> MASMTGGQQMGRDQAGITGTWYNQLGSTFIVTAGADGALTGTYESAVGNAESRYVLTGRYDSAPATDGSGTALGWTVAWKNNYRNAHSATTWSGQYVGGAEARINTQWLLTSGTTEANAWKSTLVGHDTFTKVKP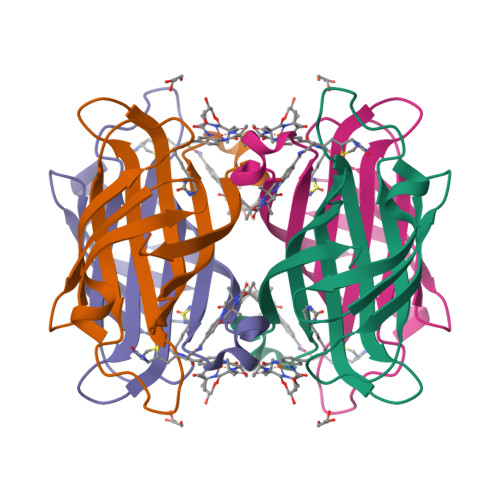SAASIDAAKKAGVNNGNPLDAVQQ>[4x]GSMTGASTTTATMRQRWQAVMMNNYGTPPIALASGDGAVVTDVDGRTYIDLLGGIAVNVLGHRHPAVIEAVTRQMSTLGHTSNLYATEPGIALAEELVALLGADQRTRVFFCNSGAEANEAAFKLSRLTGRTKLVAAHDAFHGRTMGSLALTGQPAKQTPFAPLPGDVTHVGYGDVDALAAAVDDHTAAVFLEPIMGESGVVVPPAGYLAAARDITARRGALLVLDEVQTGMG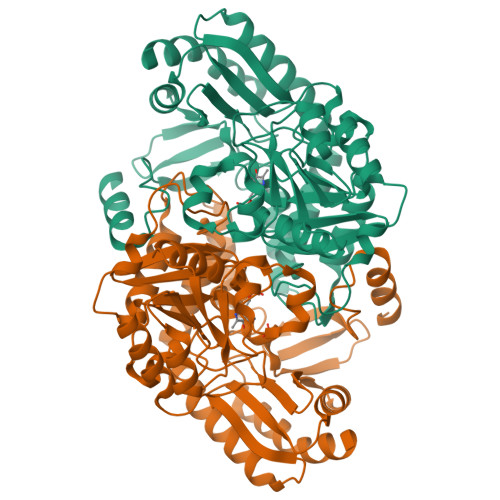RTGAFFAHQHDGITPDVVTLAKGLGGGLPIGACLAVGPAAELLTPGLHGSTFGGNPVCAAAALAVLRVLASDGLVRRAEVLGKSLRHGIEALGHPLIDHVRGRGLLLGIALTAPHAKDAEATARDAGYLVNAAAPDVIRLAPPLIIAEAQLDGFVAALPAILDRAVGAP> MANQRMLGFVHTAQRMPDKRPAAERRQDFAEIYARFSDERANEQANRCSQCGVPFCQVHCPVSNNIPDWLKLTSEGRLEEAYEVSQATNNFPEICGRICPQDRLCEGNCVIEQSTHGAVTIGSVEKYINDTAWDQGWVKPRTPSRELGLSVGVIGAGPAGLAAAEELRAKGYEVHVYDRYDRMGGLLVYGIPGFKLEKSVVERRVKLLADAGVIYHPNFEVGRDASLPELRRKHVAVLVATGVYKARDIKAPGSGLGNIVAALDYLTTSNKVSLGDTVEAYENGSLNAAGKHVVVLGGGDTAMDCVRTAIRQGATSVKCLYRRDRKNMPGSQREVAHAEEEGVEFIWQAAPEGFTGDTVVTGVRAVRIHLGVADATGRQTPQVIEGSEFTVQADLVIKALGFEPEDLPNAFDEPELKVTRWGTLLVDHRTKMTNMDGVFAA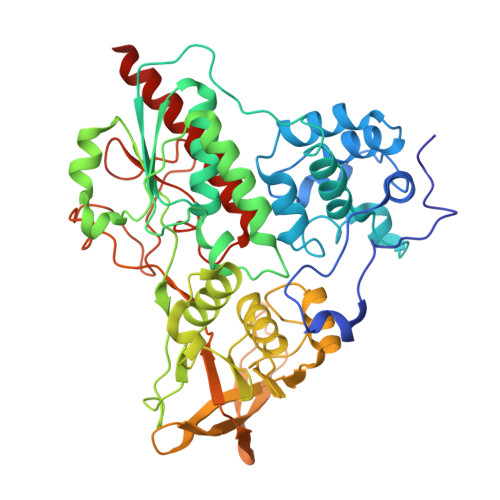GDIVRGASLVVWAIRDGRDAAEGIHAYAKAKAEAPVAVAAE> SMPPVIKIDRPFHFMIYEETSG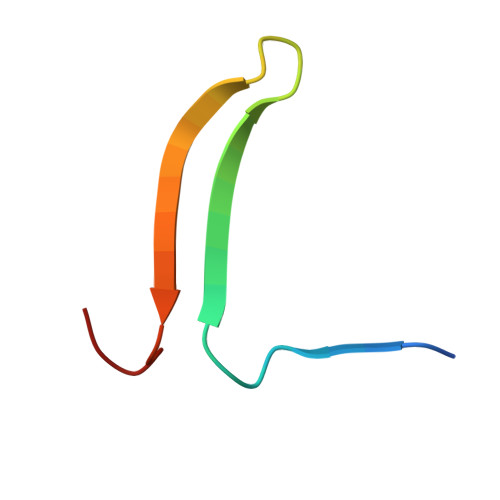MLLFLGRVVNPTLL>[4x]GPEKEWVEQ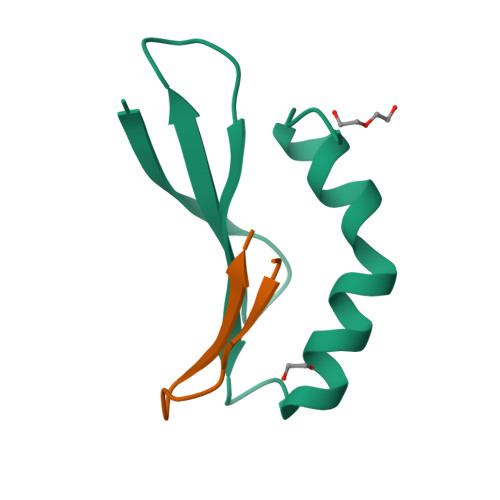DEPGVYITLTALAGGARDLKRVRFSRKRFSEIQAEQWWADNRGRVYEQYNVRMV;>GPKWVKTDSDFIVLEI[4x]>[2x]RPQGATVSLWETVQKWREYRRQC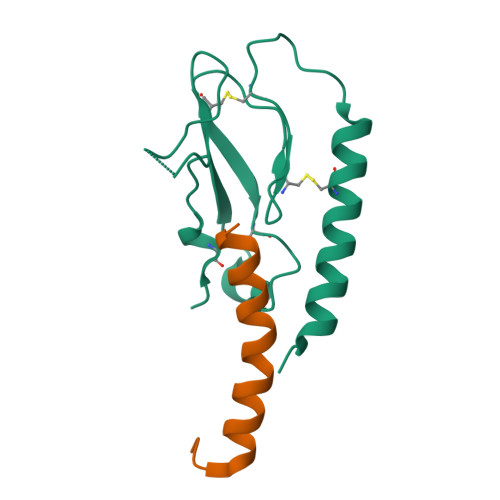QRSLTEDPPPATDLFCNRTFDEYACWPDGEPGSFVNVSCPWYLPWASSVPQGHVYRFCTAEGLWLQKDNSSLPWRDLSECEESKRGERSSPEE;>[2x]HCEGXFTSDVSSYLEGQAAKEFIAWLVKGRG CAP is a 210-amino-acid transcription factor that binds cAMP generated by adenylyl cyclase in response to the phosphorylated form of Enzyme IIAGlc (phosphorylated in response to the phosphoenolpyruvate-carbohydrate phosphotransferase system). cAMP-bound CAP regulates the transcription of over 100 genes crucial for carbon utilization through its binding to a specific promoter region and recruitment of RNA polymerase. Previous studies of the ligand binding domain of CAP demonstrated negative cooperativity between cAMP binding sites in the absence of structural change within this domain. We produce coarse-grained models that describe global low-frequency protein backbone motions of CAP and show a strong correlation between negative cooperativity for cAMP and modulation of the delocalised normal modes on ligand binding without a requirement for a spatially distinct physical pathway or conformational change. We demonstrate experimentally that altered connectivity between backbone elements in CAP can give predictable alterations to cooperativity for cAMP binding through altered mode amplitudes.

Altering local interactions associated with V140 was predicted by the ENM to have minimal effects on cooperativity despite significant local hydrophobic interactions; we therefore examined the effect of decreased and increased local hydrophobic interactions in V140A and V140L variants as a control experiment. The V140L mutant protein had no discernible effect on protein structure. As predicted by the ENM mutagenesis, measurement of cooperativity for cAMP in V140L by ITC showed no differences when compared to wild-type.

>[2x]MRGSHHHHHHGSMVLGKPQTDPTLEWFLSHCHIHKYPSKSTLIHQGEKAETLYYIVKGSVAVLIKDEEGKEMILSYLNQGDFIGELGLFEEGQERSAWVRAKTACEVAEISYKKFRQLIQVNPDILMRLSAQMARRLQVTSEKVGNLAFLDLTGRIAQTLLNLAKQPDAMTHPDGMQIKITRQEIGQIVGCSRETVGRILKMLEDQNLISAHGKTIVVYGTR2-[(2S)-6-(2-methylbut-3-en-2-yl)-7-oxo-2,3-dihydro-7H-furo[3,2-g]chromen-2-yl]propan-2-yl 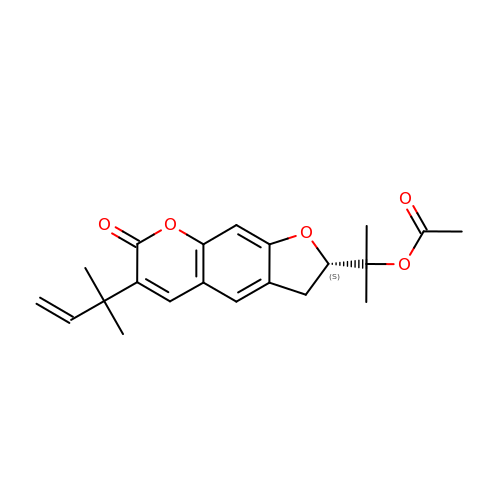acetate | C21 H24 O5 | AWMHMGFGCLBSAY-SFHVURJKSA-N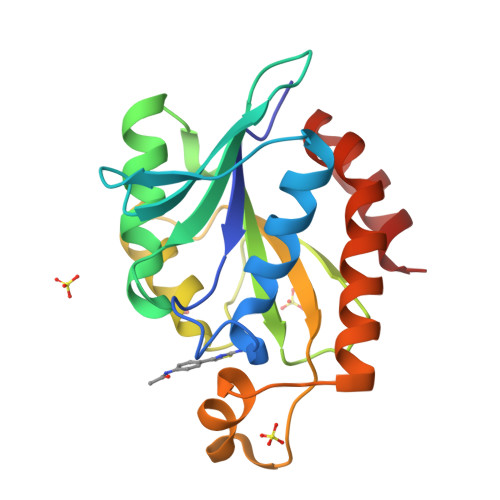>[2x]MSNTIKMVVGLGNPGKEYEQTRHNAGFWFLDELAWKWKASFKEEKKFFGEVARAALPDGDVWLLKPATFMNRSGQAVAALAQFYKIKPEEILVVHDELDIPCGRIKFKLGGGNGGHNGLKDIQAKLGTADYYRLRLGIGHPGDRNLVVGYVLNKPSAEHRRQIDDAVAKSLQAVPDIISGKWEEATRFLHSK5-chloro-1-(beta-D-glucopyranosyl)pyrimidine-2,4(1H,3H)-dione | C10 H13 Cl N2 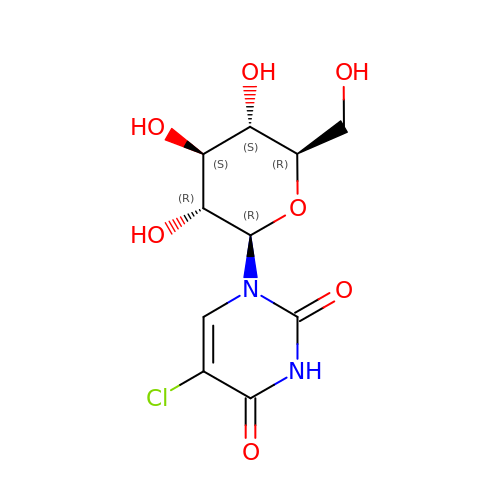O7 | NONSBAHWXCNSII-XSEHCYKFSA-N Nucleolar protein 66 (NO66) is a JmjC domain-containing protein which has been reported to be a histone demethylase and a ribosome protein 8 (Rpl8) hydroxylase. Nucleolar protein 66 (NO66) is a metazoan JmjC domain-containing protein that is highly conserved throughout evolution and was initially identified as a dual-location intranuclear protein. Evidence from a recent study indicated that NO66 hydroxylates ribosome protein 8 (Rpl8) and controls the biogenesis of the ribosome, which is consistent with the observation that NO66 is a constitutive nucleolar component. Moreover, previous work demonstrated that NO66 assembles as a tetramer and that the binding site of NO66 to osterix is located on the surface formed by a hinge region (interface I) from neighbouring subunits in the tetramer.

To gain insight into the molecular mechanisms for the enzymatic activity of NO66, we solved the crystal structure of NO66176–C in complex with Rpl8204–224 at 2.2 Å resolution. The fragment of NO66 that we used for structural analysis lacks the N-terminal 175 amino acids (referred to as NO66176–C). To determine the complex structure of NO66176–C and Rpl8204–224, Fe2+ ion and αKG were substituted by Ni2+ and NOG to prevent the reaction catalyzed by NO66 during crystallization. In the complex structure of NO66176–C and Rpl8204–224 only residues 212–222 of Rpl8 are visible in the electron-density map. In the complex structure, Rpl8204–224 forms a U-shaped conformation with a bulge-shaped structure in the middle of the peptide. In the active site of NO66, two histidine residues of the Rpl8204–224 peptide, His216 and His218, are accommodated in two deeply buried pockets. His216 is directed to the active centre by forming hydrogen bonds to Tyr328 and Ser421. The side chains of Asn215, His216 and His218 form hydrogen bonds to amino-acid residues from NO66, which determines the specificity of the recognition between NO66 and Rpl8. The distance between the active sites in the dimer linked by interface II is 1.8 Å closer in the complex structure than in NO66176–C–Ni2+.

>GGEPAWDSPLRRVLAELNRIPSSRRRAARLFEWLIAPMPPDHFYRRLWEREAVLVRRQDHTYYQGLFSTADLDSMLRNEEVQFGQHLDAARYINGRRETLNPPGRALPAAAWSLYQAGCSLRLLCPQAFSTTVWQFLAVLQEQFGSMAGSNVYLTPPNSQGFAPHYDDIEAFVLQLEGRKLWRVYRPRVPTEELALTSSPNFSQDDLGEPVLQTVLEPGDLLYFPRGFIHQAECQDGVHSLHLTLSTYQRNTWGDFLEAILPLAVQAAMEENVEFRRGLPRDFMDYMGAQHSDSKDPRRTAFMEKVRVLVARLGHFAPVDAVADQRAKDFIHDSLPPVLTDRERALSVYGLPIRWEAGEPVNVGAQLTTETEVHMLQDGIARLVGEGGHLFLYYTVENSRVYHLEEPKCLEIYPQQADAMELLLGSYPEFVRVGDLPCDSVEDQLSLATTLYDKGLLLTKMPLALN[2x];>[2x]GGGNHQHIGKP>MSAQSAVGSIETIGFPGILAAADAMVKAGRITIVGYIRAGSARFTLNIRGDVQEVKTAMAAGIDAINRTEGADVKTWVIIPRPHENVVAVLPIDF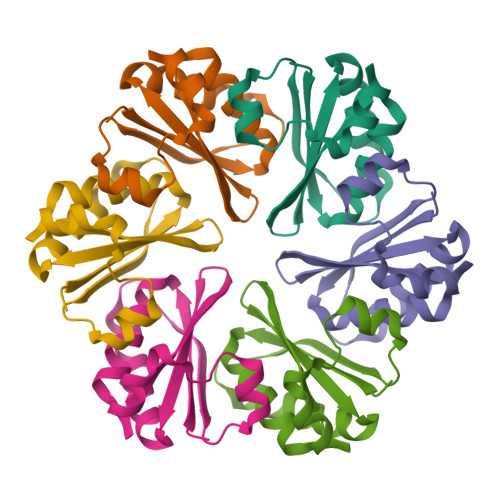SPEVEPFREAAEGLNRRGVPRGLEHHHHHH[3x]> MDTEGFGELLQQAEQLAAETEGISELPHVERNLQEIQQAGERLRSRTLTRTSQETADVKASVLLGSRGLDISHISQRLESLSAATTFEPLEPVKDTDIQGFLKNEKDNALLSAIEESRKRTFGMAEEYHRESMLVEWEQVKQRILHTLLASGEDALDFTQESEPSYISDVGPPGRSSLDNIEMAYARQIYIYNEKIVNGHLQPNLVDLCASVAELDDKSISDMWTMVKQMTDVLLTPATDALKNRSSVEVRMEFVRQALAYLEQSYKNYTLVTVFGNLHQAQLGGVPGTYQLVRSFLNIKLPAPLPGLQDGEVEGHPVWALIYYCMRCGDLLAASQVVNRAQHQLGEFKTWFQEYMNSKDRRLSPATENKLRLHYRRALRNNTDPYKRAVYCIIGRCDVTDNQSEVADKTEDYLWLKLNQVCFDDDGTSSPQDRLTLSQFQKQLLEDYGESHFTVNQQPFLYFQVLFLTAQFEAAVAFLFRMERLRCHAVHVALVLFELKLLLKSSGQSAQLLSHEPGDPPCLRRLNFVRLLMLYTRKFESTDPREALQYFYFLRDEKDSQGENMFLRCVSELVIESREFDMILGKLENDGSRKPGVIDKFTSDTKPIINKVASVAENKGLFEEAAKLYDLAKNADKVLELMNKLLSPVVPQISAPQSNKERLKNMALSIAERYRAQGISANKFVDSTFYLLLDLITFFDEYHSGHIDRAFDI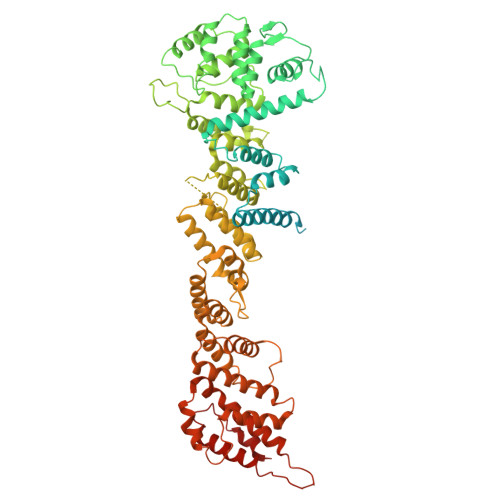IERLKLVPLNQESVEERVAAFRNFSDEIRHNLSEVLLATMNILFTQFKRLKGTSPSSSSRPQRVIEDRDSQLRSQARTLITFAGMIPYRTSGDTNARLVQMEVLMN>[4x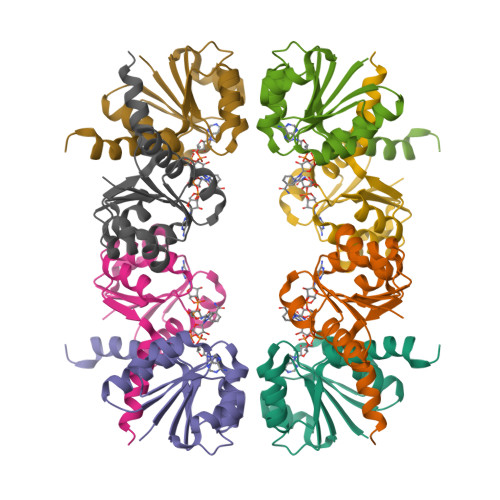]MGRIKNKQFAVIGLGRFGGSIVKELHRMGHEVLAVDINEEKVNAYASYATHAVIANATEENELLSLGIRNFEYVIVAIGANIQASTLTTLLLKELDIPNIWVKAQNYYHHKVLEKIGADRIIHPEKDMGVKIAQSLSDENVLNY>QRKNNNKRWYFTREQLENSPSRRFGLDPDKELSYRQQAANLLQDMGQRLNVSQLTINTAIVYMHRFYMIQSFTRFHRNSVAPAALFLAAKVEEQPKKLEHVIKVAHTCLHPQESLPDTRSEAYLQQVQDLVILESIILQTLGFELTIDHPHTHVVKCTQLVRASKDLAQTSYFMATNSLHLTTFSLQYTPPVVACVCIHLACKWSNWEIPVSTDGKHWWEYVDATVTLELLDELTHEFLQILEKTP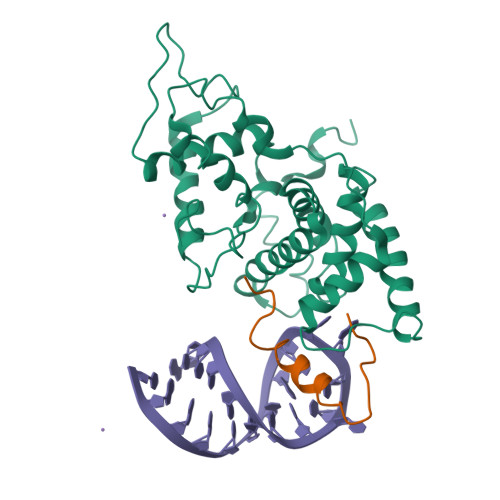NRLKRIWNWRACQAAKKT[2x];>[2x]IDYLDASLRKKNKQRLKAIQQGRQPQYLL>[2x]SNAKDDGAYKAEP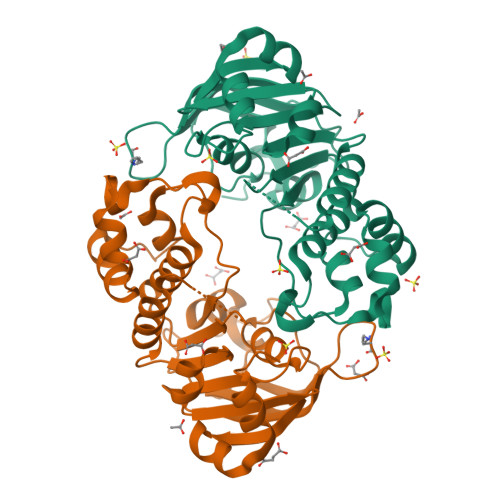AKGELEFKNVSFAYQGKEELALNNISFSVPAGKTVALVGRSGSGKSTIANLVTRFYDIEQGEILLDGVNIQDYRLSNLRENCAVVSQQVHLFNDTIANNIAYAAQDKYSREEIIAAAKAAYALEFIEKLPQGFDTVIGENGASLSGGQRQRLAIARALLRNSPVLILDEATSALDTESERAIQSALEELKKDRTVVVIAHRLSTIENADEILVIDHGEIRERGNHKTLLEQNGAYKQLHSMQFTG> MAHSSATAGPQADXSGEIAELYDLVHQGKGKDYHREAADLAALVRRHSPKAASLLDVACGTGMHLRHLADSFGTVEGLELSADMLAIARRR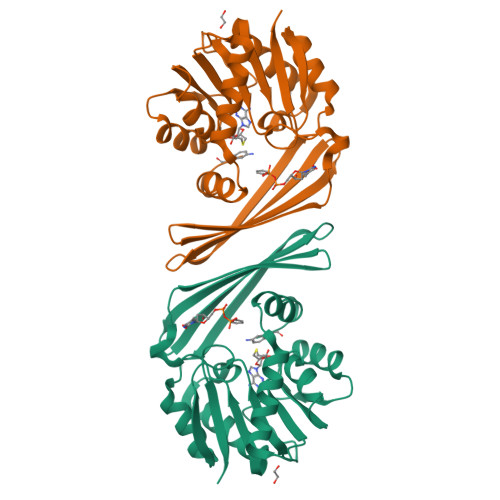NPDAVLHHGDMRDFSLGRRFSAVTCMFSSIGHLAGQAELDAALERFAAHVLPDGVVVVEPWWFPENFTPGYVAAGTVEAGGTTVTRVSHSSREGEATRIEVHYLVAGPDRGITHHEESHRITLFTREQYERAFTAAGLSVEFMPGGPSGRGLFTGLPGAKGETRLEHHHHHH>MQIQRHSFKWILYGFLCWMTSFVQAQTPTLTNATPAEGFIGEQVCFPVTFVNTGAPGYGPYVRLIVPTGFTFDNASFGGSIQTVQNLGVIVSGAPNNFVIDPIAQSNNNSTTSDTIFAPVGSTVILLEYPVGSMVQGGVSLISEVCMTVDPAATIGVPVDICTQGVYEFGDTPTGDNGPIAGANECEPIIPILFRFDKKVNGSDGVYNEVPGGGASLCHIHQYELNIDIAAAGTLNGPITITDVLPGELAYFGNISLPAGCSAVEPTVGGLGGTLTVTCNGSYPGSTANIDMQVTFDAAVSDTLDETICDDTDINNGATVNVPGNPSQSDTVVTHVEHVLLGHTNNTVSPVTIGQTVLYTIGAEITEYTAGLTAASITFIVPDGMIYNPASLTWAGTPVAAGNVVIVPGPGTGSTVTVDVHTQNGANILPCASPSLQYTADVNQTYANGDPVLSRDRLTHSSTLTYDLVEGATGCTTSAGTPIDVIDIFFQKTVNNSPPTGPGRNGQWWPGDVVQYRLELQIPSLDLDDVVITDFFPLPIHDVASLAATFGTDVRFDPATCWNTAPVTYTRDIPTNSLILDFGDVSDLVTGGCVDIVLLIDIPITTLPFADGLFHSNFMQVNSDNSTADNITNSALTLIQVGAPDLELTKGIVSSDNPNVTISPTVVPPDGNATDVSAGDQLFFDITIENVGGAPGYDVQVRDVAPPELTNCALVAPNPVVDGSNNALAFSGGFVGNTLTIDLVAPNDSIAFATAPNNNDLITVSYVCEAVAGIQAGTRFDNTAEVDWSSTRGGVKFPPVEDDANGRIADPTMNKVVDYIFPNYSNTNTQASIGEVVAYELQLNIPEGNMNNVTLVDQVDEGLAFVAVDSIVICNSSGSTNIITSIGGGFPAVQSGATITNLGANPQQQDRVLTLDFGNLQNLDTDNIEDTIKVYYRTIVINHVTNFDGERVRNRAVLSWDNPNTPGDRSSINDRAPFVTIVEPQLEISKSFTPDEVLPGNNSFVTLTVRNPGTSSAPAFDVSLTDILPTGMTFVSGFSAGGTASITTPPTNGGGTITAHWDTINVGEVYSITFEVQASSSITPCFTLTNCANLVWESIAEADEPNMPTAFSSNLGVQRTGNPGNLGGAANTYTQDSCADLDVVIDNTFDPFITANTPLCEGDRVVLTVQQYQGNVVRYNWTGPGVPAGFNNYELVLDPVTTADTGTYFVYVELDGCITDTSNFFSLQLRPKPVTPNINPGDTTICEGTSIQFSTSTIANDYTWTGPNGFTANSATTPLISPVTLADAGRYTLFTTNAQGCNSDPISSNLTVTPRPAQPSIASNTPICSNENIILTSSTSAITYQWMAPNGQDTITTNNTLTLEPNNPLYTAGNWTLVVFDANGCASQPSTAANVIINGTPIAPMTSNSGPICEGEDVTLMVNTVSSGTYAWYSDANLTNLVASTQNPVISGLLASNSPDTFYVQVSSNGCLSDTGFTVVQVNPNPAAVSPGYTPLCSGDTIFLFANATANIYNWTGPNGFVSNLENPFIANSAALNAGSYTVSITDANGCSNSGIVQVAVDERPVTPTITGNGPVCEGDNIQLNIGSYTGTTVQYTWSTPTGVVTTGVPSLNINNTTVADSGLYSVVVAVDGCTSLADSINIVVRPNPIAPNVPSNFSVCEGDGIALTTTTNANIYNWTGPNGFSSNSPNPTVISPASSANAGTYTLVVQDFNGCTSPAASTVVTVNAAPAQPSMTTNSPICNGADLVMSTSAAGNSYIWRAPNGADTTTASSTLTIVPTSSLYQSGNWTLSVVNAAGCVSPASIASAVEINSIPSTASAGNNGPVCTGTDASLSAGTVSGASYAWYTDAGTSNQFSTLQNPTVNNLTNDSTFYLLVTVNGCPSALDSTTVVVYPLTPSPSLPANFAVCEGDDIALSTSTVASSYDWSGPNGFTSNAQNPVVITNATGSNAGVYTLSIVDGNGCSSADTSVQVTVNAAPTQPSMTTNSPICNGADLVMSTSAVGNSYIWRAPNGADTTTASSTLTIVPTSSLYQSGNWTLSVVNAAGCVSPASIASAVEINSIPSTASAGNNGPVCTGTDASLSAGTVSGASYAWYTDAGTSNQFSTLQNPTVNNLTNDSTFYLLVTVNGCPSALDSTTVVVYPLTPSPSLPADFAVCEGDDIALSTSTVASSYDWSGPNGFTSNAQNPVVITNATGSNAGVYTLSIVDGNGCSSADTSVQVTVNAAPAQPSMTTNSPICNGADLVMSTSATGNSYIWRAPNGADTTTASSTLTIVPTSSLYQSGNWTLSVVNAAGCVSPASIASAVEINSIPSTASAGNNGPVCTGTDASLSAGTVSGASYAWYTDAGTSNQFSTLQNPTVNNLTNDSTFYLLVTVNGCPSALDSTTVVVYPLTPSPSLPADFAVCEGDDIALSTSTVASSYDWSGPNGFTSNAQNPVVITNATGSNAGVYTLSIVDGNGCSSADTSVQVTVNAAPTQPSMTTNSPICNGADLVMSTSAVGNSYIWRAPNGADTTTASSTLTIAPTSSLYQSGNWTLSVVNAAGCVSPASVASMVTINNGTNPTAFNNGPVCRGDAVQLNTTTINNALYEWYSDAALTNLISTQQNPTVANITTDSTFYLVVTVNGCPSSAVATTVTLHPTPATPNIPANFVVCEGETIALSTSTVASSYNWTGPNGFTSNLQNPAVIQPATTADAGSYTLFIVDANGCQSADTSVVVGVNRGPAAPVLTNNSAICDGDTLLLSTTASADTFRWISPNGIDTITTVNSLMIVPTNGTYYQSGDWTLITQVANNCPSEPSAPSSVVINSSTAAPTAFNDGPVCVGGDVTLSTPSAPGAFYQWYTDAALTNLVATTASFTAINITQDSTFYLVVTVNGCTSPAGSTVVNVIGQPSAPNVPADFEVCEGDDIILGTTTIAASYSWTGPNGFTSNLQNPAAITNASLIDSGIYRLVVTYSNGCVSADTTVRVGVNSNPPVPNIVSNGPICFGDTLVLSSSTSCGQSQWIGPNGNSQSTLGTPGGSNVLWTIGSTTSIPMNNANYLPGNWYMICIDTVTGCRSESNTINVIINANPDTPAVFNDGPVCEGGNSNLSTATVSGASYAWYSDSSLTSLVSTAQNPMIVNISTDTTWYLVVTVNGCSSVAGSTTVIVHPTPVTPNVPANFAVCEGDNITLSTSTVASSYNWSGPNGFTSNVQNPVVITNATTSNAGVYTLSIIDGNGCESGDTAVTVTVDSIPATPVLSSNSAICFGDTLELSTTALATSYEWIAPDGSRITTGTNILSISSNNSLYQSGDWMLVTTNASGCTSMPSSVATVVINANPAQPAVFNDGPVCEGGNSNLSTATVSGASYAWYSDSSLTSLVSTAQNPMIVNISTDTTWYLVVTVNGCSSVAGSTTVIVHPTPATPNVPANFAVCEGDNITLSTSTVASSYNWSGPNGFTSNVQNPVVITNATTSNAGVYTLSIVDGNGCESGDTTVTVTVDSIPVTPVLSSNSAICFGDTLELSTTALATSYEWIAPDGSRITTGTNILSISSNNSLYQSGDWMLVTTNASGCTSMPSSVATVVINANPAQPAVFNDGPVCEGGNSNLSTATVSGASYAWYSDSSLTSLVSTAQNPMIVNISTDTTWYLVVTVNGCSSVAGSTTVIVYPTPATPNVPANFAVCEGDNITLSTSTVASGYNWSGPNGFTSNVQNPVVITNATASNAGVYTLSIVDGNGCESGDTTVTVTVNGNPPVATITSNSPICFGDTLTLSSSTNCGQSQWIGPNGNSSGTLGTPGGNNVLWTIGSTTNIPSTDVNYLSGDWYMICIDTITGCRSESNTITIEINPIPVVSAFNNGPICAGEDGELSATFITGASYRWYSDATLTTLISTSRTPIISSMMSSETYYVVATVNGCTSLADSTTIVVNPTPVIPNPTYTPLCQLDTLFLQANAVGPIATYWWTGPNGFTSHLENPVIPNIYPFNAGSYILTVTDSLGCEAVSTVEVTIYPKPQTPTIAHNAPFCEGTNDLTLTTQAYFGTDVRYIWTLPNGNLDTTFVPSLVLPNATVQDTGAYSLVVWIDGCLSLPAEEIIRIYPTPATPNVPADFAVCEGEAIVLTTTTNATSYFWTGPNGFQSNLQSPSVVNATLVDAGSYHLYVTNTWGCQSLDTSVQVTVNANPPIATITSNSPICFGDTLTLSSSTNCGQSQWIGPNGNSTGTLGTPGGNNVLWTIGSTTNIPSTDSNYLSGDWYMICIDTITGCRSESNTITIDINPIPSTPAAFNNGPICIGGTAQLSTTTVSGATYAWYADATLTTLVATNQNPTISNITTDSTFYIVVTVNGCSSLAGSTTVSTYPVPATPAVPADFAVCEGDNIVLSTTTVAAGYNWTGPNGFTSNLQNPSVVSASLVDSGTYTLFIIDANGCPSGDTSVQVSVHPNPVQPVLSSNSAICDGDSLVLSTTATATTYRWVAPDGADTLTTVNTLVILPSNAFYQDGNWTLMTMDANGCQSILSNPESVTIHSIPAAQAVFNNGPVCRGSSVNLSTSFISGATYEWYADAALTILVATSQNPTINNITTDSTFYLVITVNGCTSAAGATTVVVHPTPTTPNVPSNITVCEGDAIVLTTTTNASAYVWSGPNGFSSNQQSPTVINAATVVDSGKYSLYVIDANGCRSEDTSLQVVVNPTPTTPLIVSNNTPICEGSNIVLSANAGAAGTTYEWFNASNVSVGTGQTLTIVGATVADAGDYYVITTLNSCSSAASSTTTAIVDQVPSTAAFAGNDINLCNSFTTTLDATPPNSATGFWTTNSGATIANPNLANSAVYNLPTGTSTFYWTLSNGACIDFSVDSMVVEVTPASTDVADAGLDQNLCGQTSATLTAANPSTATGQWTQSASQAGQGIVITNPTNPNTTVTGLQQGNNYTFTWTLSNGNCTDYSTDMVQINVDVSPPDNAYAGVDILLCNQNTANLDAFVSQYGTGMWTSTSSATIIDPTLANTTVINLPQDTSVFVWTLSNGTCQNYSTDSVLVVVSTTTDTAEAGNNQVVCSVNALTLGATMPSSGFGTWSQTAAQAAQGVVIVDVNDPNTQVVGLNAGTTYAFTWTLSNGTCQDYSSDVTTISVNATPPDNAFAGNDINLCGVATTTNLAASVPTVAMGLWTTTSSATISNPTQPNSTVSGLSAGQNIFIWTLSNGTCQDYDSDTVIVTVTTPSSDVADAGLDSAYCAQSVVTLNAVAPSVGGGYWSQTPSQASLGAVIDNPTDTATTVSNLMPGVTYTFTWTLTNGGCVDYSSDQVLITIDVLPTNVAYAGEDTILCGGNAVQLDGLAPPIGTGFWTTNDTATIVTPVDPNSLVVNIAEDTTTYYWTLSNGACVDYSVDSVTVIISPASTDLAFAGYDEVLCGVDSIMLSAAVPTTSTGIWTQSAGQASQGIVITNPTNPNSSVTGIQAGQVYTFTWTLSTFGCANFSTDDVQYTINALPPEVAYAGPDIVLCTGNSVTMDANNPIFSTGVWSSNSSAVIVNPTLSNSNIVNIPTDTVAFYWSLSNGSCADYSIDTMLIIVTPTFSVDTANAGLDINLCNEDTAQLMAIAPNVATGRWTQPFNQSSAGVVITDPNAAMTTATGLQLDSTYTFTWSVSNGPCRDYDRDQVIVQVSTLPTDAAYAGEDFVICGIDTAIVSATAPSIGAGMWTTTTTATIVTPPSTRTELLNLSLGSNEFIWTLSNGACRDYSSDTIVITMDSAPIANADSFVVIYNSNGNTIDVTPNDGLNNNWVITISESIASGTLDNLGTGEFDLFLQDVLVDQRFIYQLCNPNCPAIYCDTAL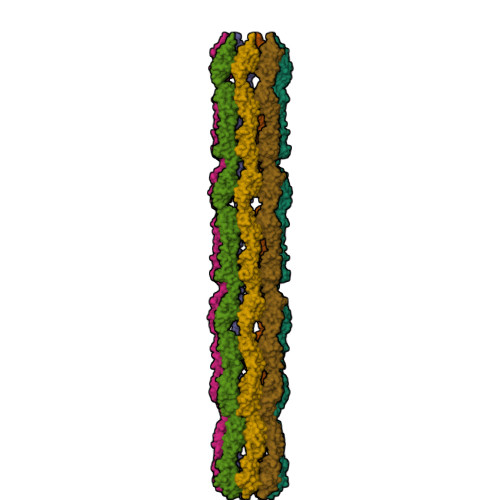VTIDVQGGTECNFPNMITPNNDDANETFIVPCLDGLEGTKFAVYNRWGDLMYENDNYKNDWGGTHNGVPVPDATYFYIMELADGQRFQGFVEVRR[7x]Arthrobacter nitroguajacolicus Rü61a 1-H-3-hydroxy-4-oxoquinaldine 2,4-dioxygenase (HOD) and Pseudomonas putida 33/1 1-H-3-hydroxy-4-oxoquinoline 2,4-dioxygenase (QDO) were the first dioxygenases discovered to belong to the ABH-fold family. They catalyze the O2-dependent breakdown of N-heteroaromatic quinolone-type substrates with concomitant carbon monoxide production. Atypical for oxygenases, these enzymes promote the activation of the triplet ground-state O2 molecule without the aid of metal centers or external organic co-factors. Kinetic measurements indicate that their reaction mechanism relies on a fast initial step, during which the substrates' 3-hydroxyl group is deprotonated by the His-Asp subset of the triad, thus promoting its activation for molecular oxygen attack (step 1), whilst the nucleophile is not essential.

The HODS101A variant was also considered interesting as the AqdC ABH-fold dioxygenase that catalyzes a chemical reaction identical to HOD naturally possesses an alanine instead of a serine at the nucleophilic elbow (hydrophobic elbow). MQO binds to HODS101A as observed with HODH251A. Although the S101A replacement causes the loss of the H-bond between S101(OG) and MQO(O4) this is compensated by the interaction with H251(NE2) resulting in an essentially identical binding mode. Under normoxic conditions, electron density at the R-site of HODS101A is consistent with the presence of a water molecule (Fig. S9†). Next to the R-site, a water molecule (W3) is also present at a H-bond distance from O1 (2.7 Å) stabilized by the side chain of H100 that is flipped compared to the HODH251A variant. W3 and H100 flipping are also seen under normoxic conditions in two of the four molecules present in the a.u. In HOD, S101A replacement, however, has a negative impact on the KM value of its organic substrate (60-fold increase compared to that of wild-type HOD) whilst kcat is not affected.

>MRGSHHHHHHGSMTDTYLHETLVFDNKLSYIDNQRDTDGPAILLLPGWCHDHRVYKYLIQELDADFRVIVPNWRGHGLSPSEVPDFGYQEQVKDALEILDQLGVETFLPVSHAHGGWVLVELLEQAGPERAPRGIIMDWLMWAPKPDFAKSLTLLKDPERWREGTHGLFDVWLDGHDEKRVRHHLLEEMADYGYDCWGRSGRVIEDAYGRNGSPMQMMANLTKTRPIRHIFSQPTEPEYEKINSDFAEQHPWFSYAKLGGPTHFPAIDVPDRAAVHIREFATAIRQGQ[4x]> MYGSKTFIKYVSGIPDYFKQSFPEGFTWERTTTYEDGGFLTAHQD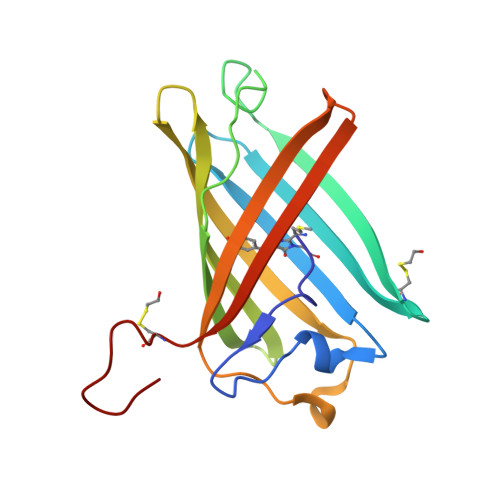TSLDGDCLVYKVKILGNNFPADGPVMQNKAGGWEPGCEILYEVDGVLCGQSLMALKCPGGRHLNCRLHTTYRSKKPASALKMPEFHFEDHRIEVKEVQKGKHYEQYEAAVARYCDAAPSKLGHH>GSTDNPDGIDYKTYDYVGVWGFSPLSNTNWFAAGSSTPGGITDWTATMNVNFDRIDNPSITVQHPVQVQVTSYNNNSYRVRFNPDGPIRDVTRGPILKQQLDWIRTQELSEGCDPGMTFTSEGFLTFETKDLSVIIYGNFKTRVTRKSDGKVIMENDEVGTASSGNKCRGLMFVDRLYGNAIASVNKNFRNDAVKQEGFYGAGEVNCKYQDTYILERTGIAMTNYNYDNLNYNQWDLRPPHHDGALNPDYYIPMYYAAPWLIVNGCAGTSEQYSYGWFMDNVSQSYMNTGDTTWNSGQEDLAYMGAQYGPFDQHFVYGAGGGMECVVTAFSLLQGKEFENQVLNKRSVMPPKYVFGFFQGVFGTSSLLRAHMPAGENNISVEEIVEGYQNNNFPFEGLAVDVDMQDNLRVFTTKGEFWTANRVGTGGDPNNRSVFEWAHDKGLVCQTNITCFLRNDNEGQDYEVNQTLRERQLYTKNDSLTGTDFGMTDDGPSDAYIGHLDYGGGVECDALFPDWGRPDVAEWWGNNYKKLFSIGLDFVWQDMTVPAMMPHKIGDDINVKPDGNWPNADDPSNGQYNWKTYHPQVLVTDMRYENHGREPMVTQRNIHAYTLCESTRKEGIVENADTLTKFRRSYIISRGGYIGNQHFGGMWVGDNSTTSNYIQMMIANNINMNMSCLPLVGSDIGGFTSYDNENQRTPCTGDLMVRYVQAGCLLPWFRNHYDRWIESKDHGKDYQELYMYPNEMDTLRKFVEFRYRWQEVLYTAMYQNAAFGKPIIKAASMYNNDSNVRRAQNDHFLLGGHDGYRILCAPVVWENSTERELYLPVLTQWYKFGPDFDTKPLEGAMNGGDRIYNYPVPQSESPIFVREGAILPTRYTLNGENKSLNTY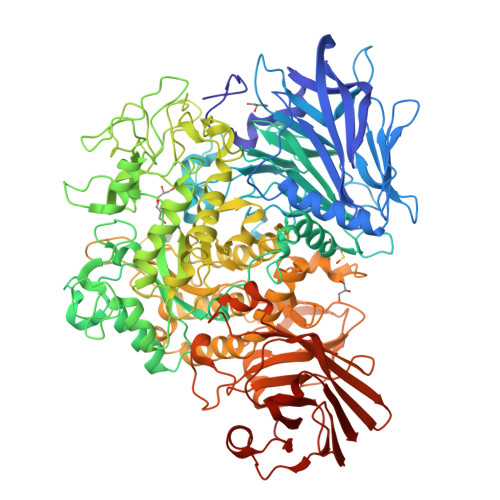TDEDPLVFEVFPLGNNRADGMCYLDDGGVTTNAEDNGKFSVVKVAAEQDGGTETITFTNDCYEYVFGGPFYVRVRGAQSPSNIHVSSGAGSQDMKVSSATSRAALFNDGENGDFWVDQETDSLWLKLPNVVLPDAVITIT[4x]>[2x]IEGGALVLHYLPEIDMRTGEVLAAE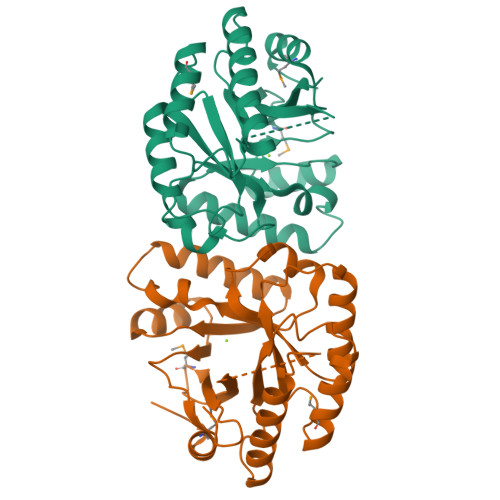ALVRWEHPTRGLLSPDSFIGVAESINLAGELGRWVLRTACAEFSRWRANGVGRNIVLRINVSPVQLVTDGFVESVAGIMKEFGLPRGSVCLEITESVVVQDIETTRTTLTGLHNVGVQVAIDDFGTGYSVLSLLKSLPVDTLKIDRSFVAELGSNPGDLPIVRAVIALAGAFGLQLVAEGVETERAALTLLRHGCYRAQGFLLSKPILGSEMQTLLAKGRVP>MERSALVTGGASGLGRAAALALKARGYRVVVLDLRREGEDLIYVEGDVTREEDVRRAVARAQEEAPLFAVVSAAGVGLAEKILGKEGPHGLESFRRVLEVNLLGTFNVLRLAAWAMRENPPDAEGQRGVIVNTASVAAFEGQIGQAAYAASKGGVVALTLPAARELAGWGIRVVTVAPGLFDTPLLQGLPEKAKASLAAQVPFPPRLGRPEEYAALVL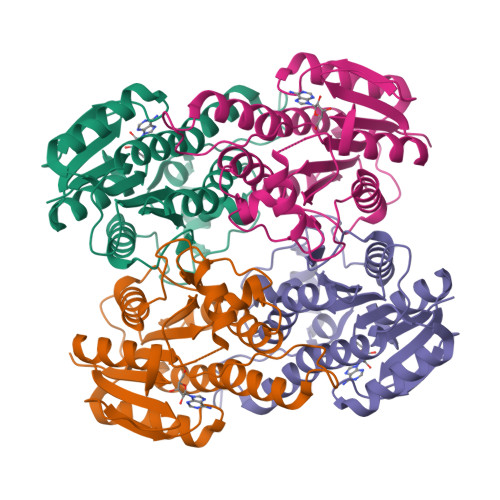HILENPMLNGEVVRLDGALRMAPR[2x]>[2x]TVEQIFDERYPLDKWKDSNYSILDKFSMRGRKGFVTGAAGGLGRNAAAALAQAGADVALVDLPSQEDKLTELAKDMSERFGTNVIALTCDVTDTVQVAELKTQLVEQLGTVDFAFLNAGVNVPGDDQDATEEVWTRTININLNGTYRTGRIAHEIMREHGHGGSLIFTASLSGHNANYMMGSPTPVNAYGATKAAIMEHSRYLAAALAKDGIRSNTISPGYVWSGIFNGRID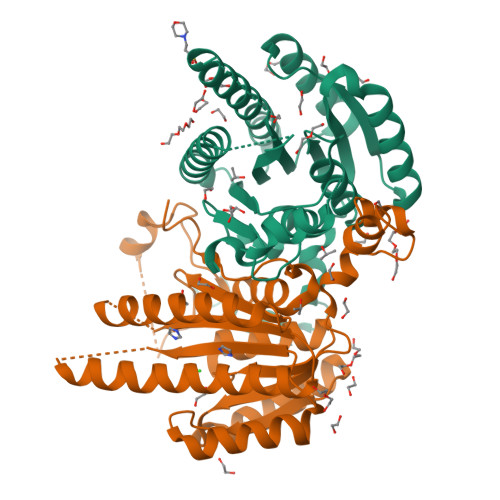MPGHDAMLEVVPMHRFGTNDEIASTVLFLASDASSYVTGTDIRVDGGYSVF>MKMTSIQQRAELHRQIWQIANDVRGSVDGWDFKQYVLGALFYRFISENFSSYIEAGDDSICYAKLDDSVITDDIKDDAIKTKGYFIYPSQLFCNVAAKANTNDRLNADLNSIFVAIESSAYGYPSEADIKGLFADFDTTSNRLGNTVKDKNARLAAVLKGVEGLKLGDFNEHQIDLFGDAYEFLISNYAANAGKSGGEFFTPQHVSKLIAQLAMHGQTHVNKIYDPAAGSGSLLLQAKKQFDNHIIEEGFFGQEINHTTYNLARMNMFLHNINYDKFDIKLGNTLTEPHFRDEKPFDAIVSNPPYSVKWIGSDDPTLINDERFAPAGVLAPKSKADFAFVLHALNYLSAKGRAAIVCFPGIFYRGGAEQKIRQYLVDNNYVETVISLAPNLFFGTTIAVNILVLSKHKTDTNVQFIDASELFKKETNNNILTDAHIEQIMQVFASKEDVAHLAKSVAFETVVANDYNLSVSSYVEAKDNREIIDIAELNAELKTTVSKIDQLRKDIDAIVAEIEGCEVQK[2x];>[2x]MDDMQVYIANLGKYNEGELVGAWFTFPIDFEEVKEKIGLNDEYEEYAIHDYELPFTVDEYTSIGELNRLWEMVSELPEELQSELSALLTHFSSIEELSEHQEDIIIHSDCDDMYDVARYYIEETGALGEVPASLQNYIDYQAYGRDLDLSGTFISTNHGIFEIVY;> MTHQTHTIAESNNFIVLDKYIKAEPTGDSYQSESDLERELIQDLRNQGYEFISVKSQSAMLANVREQLQNLNGVVFNDSEWRRFTEQYLDNPSDGILDKTRKIHIDYICDFIFDDERLENIYLIDKKNLMRNKVQIIQQFEQAGSHANRYDVTILVNGLPLVQIELKKRGVAIREAFNQIHRYSKESFNSENSLFKYLQLFVISNGTDTRYFANTTKRDKNSFDFTMNWAKSDNTLIKDLKDFTATCFQKHTLLNVLVNYSVFDSSQTLLVMRPYQIAATERILWKIKSSFTAKNWSKP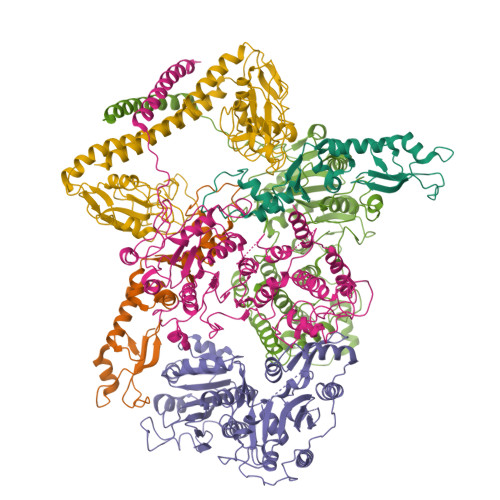ESGGYIWHTTGSGKTLTSFKAARLATELDFIDKVFFVVDRKDLDYQTMKEYQRFSPDSVNGSENTAGLKRNLDKDDNKIIVTTIQKLNNLMKAESDLPVYNQQVVFIFDECHRSQFGEAQKNLKKKFKRYYQFGFTGTPIFPENALGSETTASVFGRELHSYVITDAIRDEKVLKFKVDYNDVRPQFKSLETETDEKKLSAAENQQAFLHPMRIQEITQYILNNFRQKTHRTFPGSKGFNAMLAVSSVDAAKAYYATFKRLQEEAANKSATYKPLRIATIFSFAANEEQNAIGEISDETFDTSAMDSSAKEFLDAAIREYNSHFKTNFSTDSNGFQNYYRDLAQRVKNQDIDLLIVVGMFLTGFDAPTLNTLFVDKNLRYHGLMQAFSRTNRIYDATKTFGNIVTFRDLERSTIDAITLFGDKNTKNVVLEKSYTEYMEGFTDAATGEAKRGFMTVVSELEQRFPDPTSIESEKEKKDFVKLFGEYLRAENILQNYDEFATLKALQQIDLSDPVAVEKFKAEHYVDDEKFAELQTIRLPADRKIQDYRSAYNDIRDWQRREKEAEKKEKSTTDWDDVVFEVDLLKSQEINLDYILGLIFEHNRQNKGKGEMIEEVKRLIRSSLGNRAKEGLVVDFIQQTNLDDLPDKASIIDAFFTFAQREQQREAEALIKEENLNEDAAKRYIRTSLKREYATENGTELNETLPKLSPLNPQYKTKKQAVFQKIVSFIEKFKGVGGKI;> MSEMSYLEKLLDGVEVEWLPLGEITKYEQPTKYLVKAKDYHDTYTIPVLTAGKTFILGYTNETHGIYQASKAPVIIFDDFTTANKWVDFDFKAKSSAMKMVTSCDDNKTLLKYVYYWLNTLPSEFAEGDHKRQWISNYSQKKIPIPCPDNPEKSLAIQSEIVRILDKFTALTAELTAELNMRKKQYNYYRDQLLSFKEGEVEWKTLGEIGKWYGGGTPSKNKIEFWENGSIPWISPKDMGRTLVDSSEDYITEEAVLHSSTKLIPANSIAIVVRSSILDKVLPSALIKVPATLNQDMKAVIPHENILVKYIYHMIGSRGSDILRAAKKTGGSVASIDSKKLFSFKIPVPNINEQQRIVEILDKFDTLTNSITEGLPREIELRQKQYEYYRDLLFSFPKPETVSN> MGSDKIHHH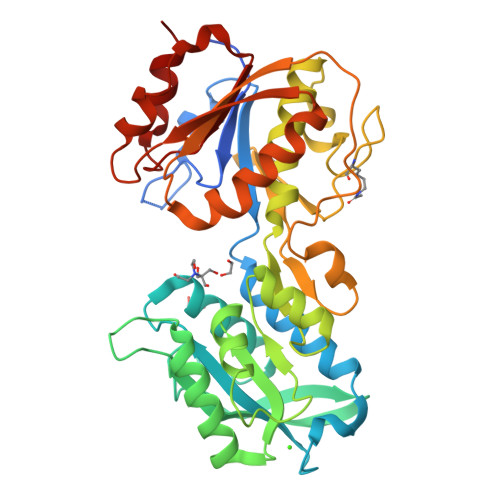HHHENLYFQGRDKPLVFFNRQPSDPLTGKVDMAAMNWNDKTYYVGFDAKFGGSIQGKMILDFLASSESSVDRNGDGIIGYVLCIGDVGHNDSKVRTEGIRRALGTWTGSSDPGQAKEGQAVVGGKSYKVVELEGKAMTGTDGSTWNTNSATESMGSWVAKFADKIDLVISNNDGMAMGCLQASNYPRGLPIFGYDANADAVESVGKGELTGTVSQNVDAQAVAVLQIIRNLLDGSSGEDVVANGISRPDAHGNKISAPVQYWEDVKAIMADNSEVTSANWKEYTRGARDAGVRQVSAPTKKVLLTVHNASNDFLASAYLPALKHYAPLLNVDLTVVQGDGQNELSCLDKFTNLDMFDAFAVNMVKTNSGADYTDKLKY> GSFVEMVDNLRGKSGQGYYVEMTVGSPPQTLNILVDTGSSNFAVGAAPHPFLHRYYQRQLSSTYRDLRKGVYVPYTQGKWEGELGTDLVSIPHGPNVTVRANIAAITESDKFFINGSNWEGILGLAYAEIARPDDSLEPFFDSLVKQTHVPNLFSLQLCGAGFPLNQSEVLASVGGSMIIGGIDHSLYTGSLWYTPIRREWYYEVIIVRVEINGQDLKMDCKEYNYDKSIVDSGTTNLRLPKKVFEAAVKSIKAASSTEKFPDGFWLGEQLVCWQAGTTPWNIFPVISLYLMGEVTNQSFRITILPQQYLRPVEDVATSQDDCYKFAISQSSTGTVMGAVIME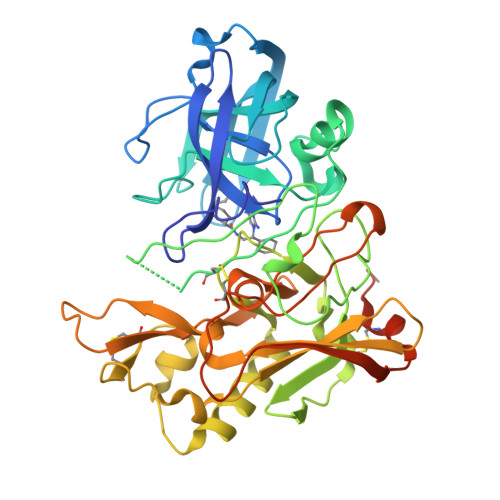GFYVVFDRARKRIGFAVSACHVHDEFRTAAVEGPFVTLDMEDCGYNIPQTDESTLMTIAYGDLHHHHHH(3~{R})-3-[[1-(2-hydroxyethyl)-5-[(4-methoxynaphthalen-1-yl)methyl]-6,7-dihydro-4~{H}-pyrazolo[4,3-c]pyridin-3-yl]carbonylamino]-3-phenyl-propanoic 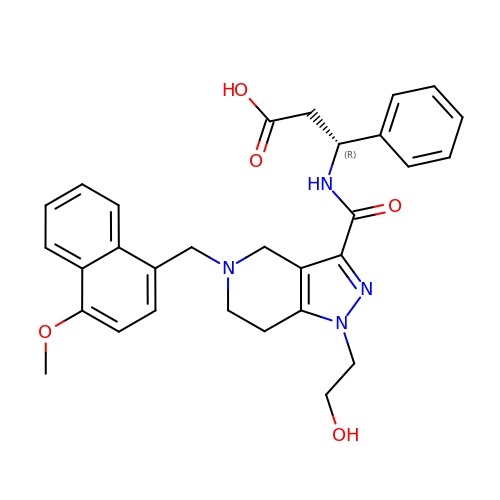acid | C30 H32 N4 O5 | FEINFPMXJVPOSJ-RUZDIDTESA-N>MRGSHHHHHHGSMEEYYMKLALDLAKQGEGQTESNPLVGAVVVKDGQIVGMGAHLKYGEAHAEVHAIHMAGAHAEGADIYVTLEPCSHYGKTPPCAELIINSGIKRVFVAMRDPNPLVAGRGISMMKEAGIEVREGILADQAERLNEKFLHFMRTGLPYVTLKAAASLDGKIATSTGDSKWITSEAARQDAQQYRKTHQSILVGVGTVKADNPSLTCRLPNVTKQPVRVILDTVLSIPEDAKVICDQIAPTWIFTTARADEEKKKRLSAFGVNIFTLETERIQIPDVLKILAEEGIMSVYVEGGSAVHGSFVKEGCFQEIIFYFAPKLIGGTHAPS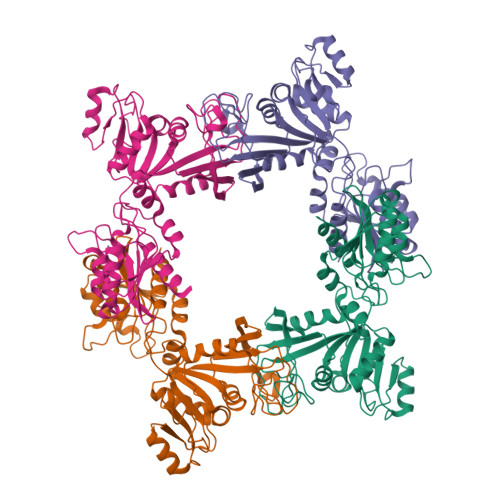LISGEGFQSMKDVPLLQFTDITQIGRDIKLTAKPTKE[4x]[[(2~{R},3~{S},4~{R},5~{R})-5-[2,6-bis(azanyl)purin-9-yl]-3,4-bis(oxidanyl)oxolan-2-yl]methoxy-oxidanyl-phosphoryl]methylphosphonic 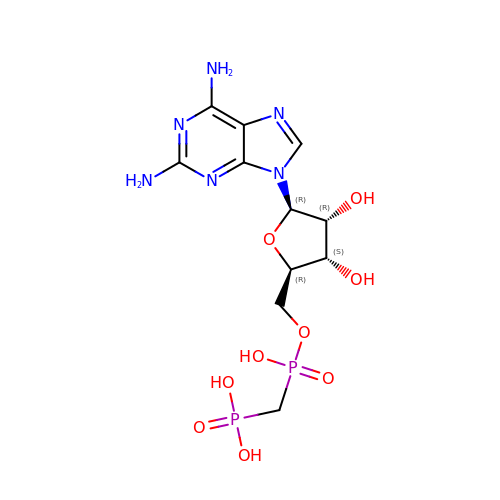acid | C11 H18 N6 O9 P2 | YUBQMXICWXUXRX-KQYNXXCUSA-N> MITTPLVHVASVEKGRSYEDFQKVYNAIALKLREDDEYDNYIGYGPVLVRLAWHISGTWDKHDNTGGSYGGTYRFKKEFNDPSNAGLQNGFKFLEPIHKEFPWISSGDLFSLGGVTAVQEMQGPKIPWRAGRVDTPEDTTPDNGRLPDADKDAGYVRTFFQRLNMNDREVVALMGAHALGKTHLKNSGYEGPWGCANNVFTNEFYLNLLNEDWKLEKNDANNEQWDSKSGYMMLPTDYSLIQDPKYLSIVKE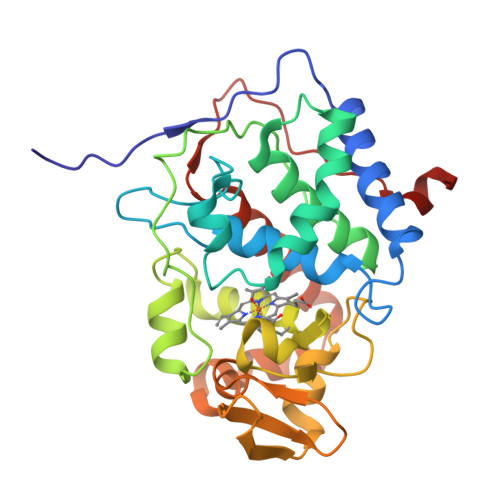YANDQDKFFKDFSKAFEKLLENGITFPKDAPSPFIFKTLEEQGL A tetratricopeptide repeat (TPR) motif containing mitochondrial outer membrane protein, mitochondrial fission protein 1 (Fis1), mediates mitochondrial fission by recruiting large cytosolic GTPase, Drp1, to the mitochondrial outer membrane. The cytosolic domain of Fis1 is composed of 6 tight α-helices with two anti-parallel TPR motifs forming a concave hydrophobic surface. Fis1 interaction with Drp1 occurs during cellular stress, but not under physiological conditions, suggesting that cellular signals during stress activate Fis1. Human Fis1 protein contains a single cysteine, Cys41, in the entire protein.

To explore this possibility further, we crystallized and determined the X-ray structures of the WT and three phosphorylation mimic-mutants of Fis1: Thr34Asp Fis1, Thr34Glu Fis1 and Tyr38Glu Fis1. Each of these mutants was previously shown to be sufficient to increase Drp1 recruitment to mitochondria and subsequent mitochondrial fission in cell-based studies. Consistently, we observed that the first 30 residues including the α1 helix were missing from the structure providing strong evidence that the α1 helix undergoes significant conformational change and is potentially disordered in the phosphorylated forms, whereas it was intact in the WT. In one of the instances, Tyr38Glu Fis1 mutant was crystallized in an intermediate state, where the α1-helix was still intact, but was shifted away from the rest of the protein, as compared to the WT. We crystallized the phosphorylation-mimic mutants, Thr34Asp, Thr34Glu and Tyr38Glu Fis1, and we observed that in all the cases, these mutants crystallized as covalent dimers mediated by Cys41 disulfide bridge between two Fis1 protomers. As Thr34Asp, Thr34Glu and Tyr38Glu Fis1 have a greater propensity for a conformationally altered N-terminus and hence have more exposed Cys41, they crystallized as covalent dimers. Upon closer examination of the crystal structures, we observed that the concave hydrophobic surface in the covalent dimers of all the phosphorylation-mimic mutants was exposed. Here we showed that Cys41 is also oxidizable and mediates Fis1 covalent dimerization through disulfide linkage. This oxidation-induced Fis1 dimerization was obvious in the crystal structures of Thr34Asp, Thr34Glu and Tyr38Glu Fis1, where we saw a clear electron density for the disulfide linkage.

>MEAVLNELVSVEDLLKFEKKFQSEKAAGSVSKSTQFEEAWCLVRSKYNDDIRKGIVLLEELLPKGSKEEQRDYVFYLAVGNYRLKEYEKALKYVRGLLQTEPQNNQAKELERLIDKAMKKDGLLEVLFQ[2x]> MAHHHHHHMSLIVTRFAPSPTGYLHIGGLRTAIFNYLFARANQGKFFLRIEDTDLSRNSIEAANAIIEAFKWVGLEYDGEILYQSKRFEIYKEYIQKLLDEDKAYYCYMSKDELDALREEQKARKETPRYDNRYRDFKGTPPKGIEPVVRIKVPQNEVIGFNDGVKGEVKVNTNELDDFIIARSDGTPTYNFVVIVDDALMGITDVIRGDDHLSNTPKQIVLYKALNFKIPNFFHVPMILNEEG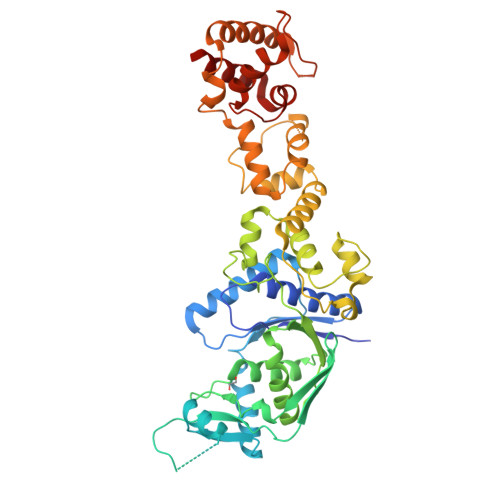QKLSKRHGATNVMDYQEMGYLKEALVNFLVRLGWSYQDKEIFSMQELLECFDPKDLNSSPSCFSWHKLNWLNAHYLKNQSAQKLLELLKPFSFSDLSHLNPAQLDRLLDALKERSQTLKELALKIDEVLIAPVEYEEKVFKKLNQALIMPLLEKFKLELKEANFNDESALENAMHKIIEEEKIKAGSFMQPLRLALLGKGGGIGLKEALFILGKTESVKRIENFLKN> LKESPSGYLRSGEGDTGCGELVWVGEPLTLRTAETITGKYGVWMRDPKPTYPYTQETTWRIDTVGTDVRQVFEYDIISQFMQGYPSKVHILPRPLESTGAVVYSGSLYFQGAESRTVIRYELNTETVKAEKEIPGAGYHGQFPYSWGGYTDIDLAVDEAGLWVIYSTDEAKGAIVLSKLNPENLELEQTWETNIRKQSVANAFIICGTLYTVSSYTSADATVNFAYDTGTGISKTLTIPFKNRYKYSSMIDYNPLEKKLFAWDNLNMVTYDIKLSKM

Inherited missense mutations in the myocilin (MYOC) gene, within its olfactomedin (OLF) domain, constitute the strongest genetic link to primary open-angle glaucoma via a toxic gain of function, and thus MYOC is an attractive precision-medicine target. Myocilin has no known function, and there is no glaucoma phenotype in Myoc knockout mice or in individuals with a homozygous N-terminal truncation mutation or hemizygous deletion of MYOC, but rare non-synonymous coding mutations lead to toxic intracellular sequestration of misfolded myocilin. However, not all mutations in MYOC cause glaucoma, and common variants are expected to be neutral polymorphisms. Among the common features associated with pathogenic myocilin misfolding, we demonstrate that a single metric, OLF thermal stability, can robustly segregate benign from early-onset disease variants.

Overall, nine variants (T256M, R296H, L303I, S313F, V329M, S331L, E352K, A427T, and V499I) were considered likely to be benign. Assessment of spent media from cells expressing each of the 16 full-length myocilin variants revealed WT-like secretion for T256M, R296H, L303I, S313F, V329M, S331L, T353I, A445V, V449I and K500R. Structural integrity was further confirmed by high-resolution crystal structures, which were solved for 11 OLF variants. No gross changes from WT OLF were detected for the structures of T293K, R296H, L303I, V329M, S331L, E352K, T353I, K398R, A445V, V449I or K500R, indicating that these mutations are accommodated within the native five-bladed β-propeller fold and do not perturb the dinuclear calcium-containing site. In addition to the five variants that we predicted initially to be benign (T293K, T353I, K398R, A445V and K500R), our study reveals seven more (T256M, R296H, L303I, V329M, S331L, E352K and V499I) that are indistinguishable from WT OLF across multiple assays. Thus, our data indicate these should also be considered benign.> GTITSQDDNVVVGYWHNWCDGRGYQGGNAPCVELKTVNPQYNVVNISFMKVYDIAEGRIPTFKLDPTIALSEAEFIAQIDTLNSQGRSVLIALGGADAHIELTRGDEDALAAEIIRLTDLYGFDGLDIDLEQAAITAKDNQFVIPAALKMVKEHYRKTGDNFMITMAPEFPYLTANGAYTPYLTELDGYYDFINPQFYNQGGDGLWIEGVGWIAQNNDALKEEFIYYIADSLINGTRNYHKIPHDKLVFGLPSNIDAAATGYIQDPQDLYKAFDRLKAQGQPLRGVMTWSVNWDMGTDAANNSYNQQFIKDYGNFIHNQLPPVTDMTPTLSGIVDTRVELDSHFDPLIGITAKDYQGNDITADVTVSGSVNTNQVGDYLLTYSVSSDDETTNQPRKITVYEILPAFTGITDTTVVIDSEFDPMQGVSASHPTQGDLTANITVTGEVDTNVVGVYELTYQLFYGQDN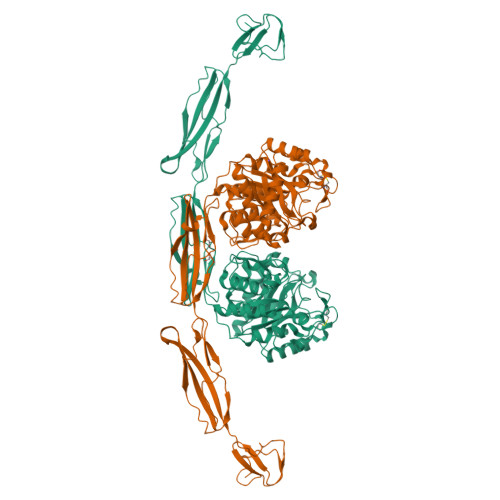QQNMTDKRIVTVVTDAVSDDDWQVGSTYVKDDKVTHNGATWTAQWWTKGEEPGTTGEWGVWR> MSAIKPDMKIKLRMEGNVNGHHFVIDGDGTGKPFEGKQSMDLEVKEGGPLPFAFDILTTAFAYGNRVFAKYPDNIQDYFKQSFPKGYSWERSLTFEDGGICNARNDITMEGDTFYNKVRFYGTNFPANGPVMQKKTLKWEPSTEKMYVRDGVLTGDVETALLLEGNAHYRCDFRTTYKAKEKGVKLPGAHFVDHCIEILSHDKDYNKVKLYEHAVAHSGLPN;> MSAIKPDMKIKLRMEGNVNGHHFVIDGDGTGKPFEGKQSMDLEVKEGGPLPFAFDILTTAFXNRVFAKYPDNIQDYFKQSFPKGYSWERSLTFEDGGICNARNDITMEGDTFYNKVRFYGTNFPANGPVMQKKTLKWEPSTE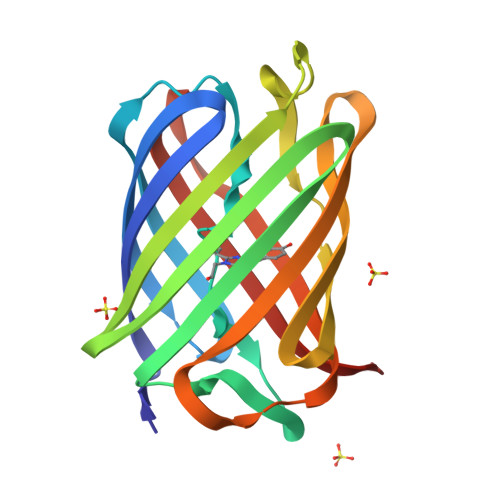KMYVRDGVLTGDVETALLLEGNAHYRCDFRTTYKAKEKGVKLPGAHFVDHCIEILSHDKDYNKVKLYEHAVAHSGLPN> MDGIAELTGARVEDLAGMDVFQGCPAEGLVSLAASVQPLRAAAGQVLLRQGEPAVSFLLISSGSAEVSHVGDDGVAIIARALPGMIVGEIALLRDSPRSATVTTIEPLTGWTGGRGAFATMVHIPGVGERLLRTARQRLAAFVSPIPVRLADGTQLMLRPVLPGDRERTVHGHIQFSGETLYRRFMSARVPSPALMHYLSEVDYVDHFVWVVTDGSDPVADARFVRDETDPTVAEIAFTVADAYQGRGIGSFLIGALSVAARVDGVERFAARMLSDNVPMRTIMDRYGAVWQREDVGVITTMIDVPGPG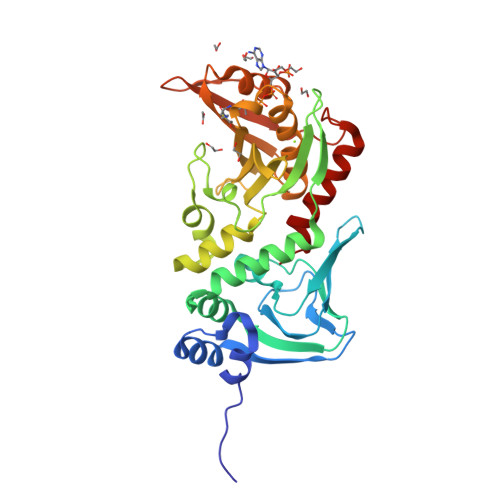ELSLGREMVDQINRVARQVIEAVG>MSLARPLSFHEDRLFPSDPATRSYARGLYALVKDLPIISPHGHTDPSWFATNAPFQDATDLLLAPDHYLFRMLYSQGVSLDALKVRSKAGVPDTDPREAWRVFASHFYLFRGTPSWVWLNHVFSQVFGFTEFLEASNADDYFDRITAALATDAFRPRALFDRFNIETLATTEGPHESLQHHAAIRESGWGGHVITAYRPDAVIDFEDERSPRAFERFAETSGQDVYSWKSYLEAHRLRRQAFIDAGATSSDHGHPTAATADLSDVEAEALFNSLVKGDVTPEKAELFR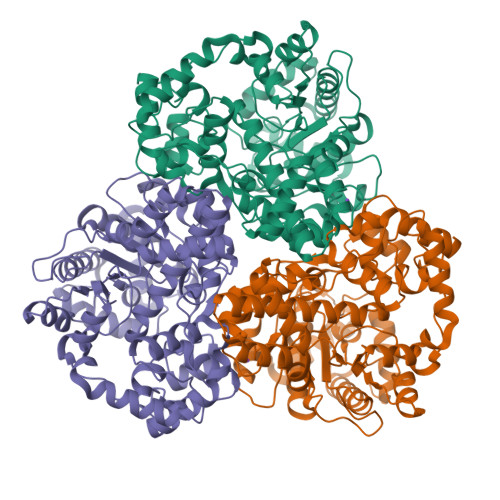AQMLTEMAKMSLDDGLVMQIHPGSHRNHNVGLLNSHGRDKGADIPMRTEYVDALKPLLTRLGNDPRLSIILFTLDETTYSRELAPLAGHYPVLKLGPSWWFHDSPEGMMRFREQVTETAGFYNTVGFNDDTRAFLSIPARHDVARRVDSAFLARMVAEHRMDLVEAEELIVDLTYNLPKKAYKLDQRPDWARPATLRAAAEEGHHHHHH[3x]HEPTANAMIDE | C7 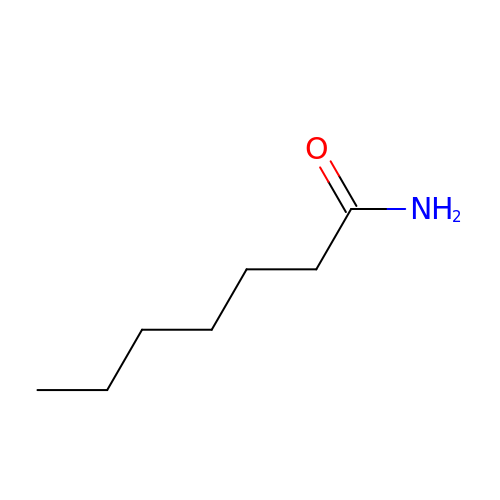H15 N O | AEDIXYWIVPYNBI-UHFFFAOYSA-N> AETKNFTDLVEATKWGNSLIKSAKYSSKDKMAIYNYTKNSSPINTPLRSANGDVNKLSENIQEQVRQLDS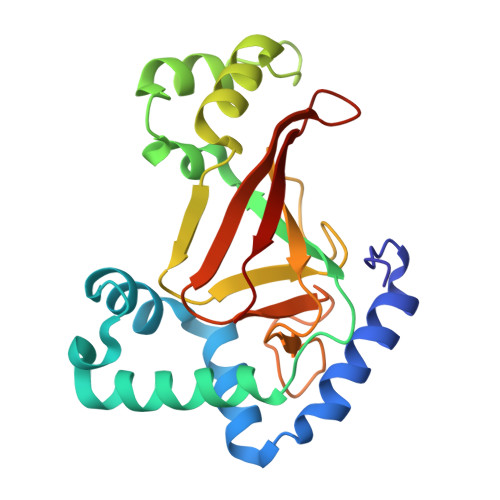TISKSVTPDSVYVYRLLNLDYLSSITGFTREDLHMLQQTNNGQYNEALVSKLNNLMNSRIYRENGYSSTQLVSGAALAGRPIELKLELPKGTKAAYIDSKELTAYPGQQEVLLPRGTEYAVGSVKLSDNKRKIIITAVVFKK Dinuclear monooxygenases mediate challenging C–H bond oxidation reactions throughout nature. The protein components of AibH1H2 stem from a largely uncharacterized structural superfamily, PF04909, containing over 100,000 unique proteins that can individually function as either carboxylases, hydratases, hydrolases, or monooxygenases. Representatives of the latter enzyme class—collectively defined here as “amidohydrolase-related dinuclear oxygenases” (AROs)—include PtmU313 and AibH2,9,15 which employ dinuclear cofactors with different metal identities. Herein we utilize this “guilt by association” strategy to identify four candidate AROs that can each harbor redox-active dinuclear active sites. Each of the four candidate AROs can harbor redox-active diiron cofactors.

The genomic neighborhoods of candidate AROs stemming from Litorilinea aerophila (A0A540VG95, referred to as SfbO), Afipia carboxidovorans (B6JH23), Cytobacillus firmus (W7L2Y2), and Geobacillus strain Y412MC10 (D3EI84) intimate disparate physiological functions. Each of these proteins was fused to an N-terminal His6 tag, recombinantly expressed in Escherichia coli, and purified as soluble protein preparations. For initial studies, the expression medium was supplemented with additional FeII sources to ensure the formation of an intact dinuclear active site. Aerobic samples of these Fe2-metalated proteins were found to exhibit moderately intense UV/vis features centered near ∼350 nm, consistent with charge transfer bands classically associated with diferric FeIII–OHx–FeIII motifs. These features were diminished upon anaerobic addition of ∼1.2 equiv of sodium dithionite (DT) and returned following reexposure of these samples to air.

>[4x]MDDTKIIDVDVHNEQDDRALLPYLQEPWRSRVAASGIGYAGSGYYSPIGVMKKDSIPPGGGKAGSDPDYMIKQLIEGYNLDYAVLTGVVYNISSTHDPDYAAAICSAYNDYLIAEWLGKHKAFKGALAVATQDPLLAAREIDRIGGHPDIVEVMISSAARSPLGQRHYHPIYEAAARNGLPVAIHPGAEGGGSSTAPTAAGYPTRYIEWHTCLSQMFMAHLVSMVCEGVFVKYPNLKVVLVEGGVAWLPGLMWRLDKNYKALRATVPWLTRMPSEYIRDHCYLSTQPIEEPDNPQHLIDLFNMIDAENMLLYSSDYPHWDFDSPGHVLRGLKPEARRKIFYENAKQLYRLD> KVFERCELARTLKRLGMDGYRGISLANWMCLAKWESGYNTRATNYNAGDRSTDYGIFQINSRYWCNDGKTPGAVNAA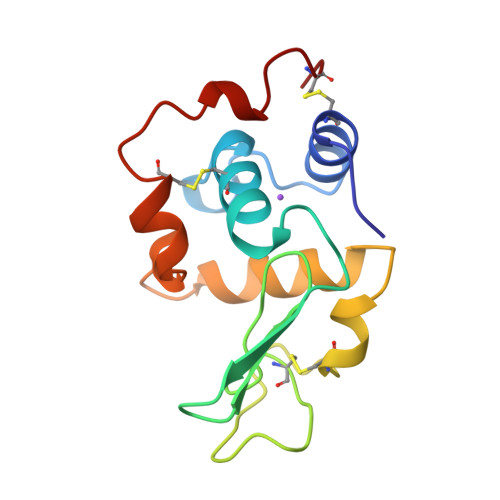HLSCSALLQDNIADAVAAAKRVVRDPQGIRAWVAWRNRCQNRDVRQYVQGCGV PUF proteins, named for PUM (Pumilio) and FBF (fem-3 binding factor), are an exemplary system for understanding the divergence of RNA recognition within eukaryotic RNA-binding protein families. Eight PUM repeats are arranged in a crescent shape with the RNA bound on the concave face of the protein. Each repeat contributes a trio of amino acid residues, termed a tripartite recognition motif (TRM), that directly contact the opposing RNA base. FBF recognizes a 9-nt motif, 5´-UGURNNAUA-3´, whereas PUF-8 binds an 8-nt sequence, 5´-UGUANAUA-3´.

A crystal structure of the AS/Y variant in complex with PBE RNA was nearly identical to the SS/Y structure. We also tested the binding preferences of an FBF-2 R5 AQ/Y variant that we identified as an in vivo substitution by genome engineering (see below). We did, however, recover multiple strains with deletion mutations and a single strain that incorporated a novel repeat R5 TRM variant - AQ/Y. This mutant strain was designated fbf-2(lot14). Serendipitously the AQ/Y mutation preferentially binds to the PBE relative to the FBE in cells and in vitro, and a crystal structure of the FBF-2 R5 AQ/Y variant bound to the PBE adopts a similar conformation to SS/Y and AS/Y bound to the PBE. The R5 AQ/Y variant displayed preference for A4, although not as strictly as PUF-8. The AQ/Y variant is most similar to the WT TRM, which seems to impart preference for A4. Finally, the FBF-2 R5 AQ/Y variant demonstrates a recognition pattern qualitatively more similar to PUF-8 than FBF-2. In the case of changing specificity of FBF-2 to that of PUF-8, we have demonstrated that a minimum of two amino acid changes (CQ/R to AQ/Y) can swap binding element length preference, but they do not impact curvature. We found that the edited strain expressing the FBF-2 AQ/Y variant (fbf-2(lot-14), glp-1(ar202) animals) displayed tumor formation in only 36% of gonads at 15°C. Thus, the FBF-2 AQ/Y variant is capable of substituting for PUF-8 in vivo.

> GSNNVLPTWSLDSNGEMRSRLSLSEVLDSGDLMKFAVDKTGCQFLEKAVKGSLTSYQKFQLFEQVIGRKDDFLKLSTNIFGNYLVQSVIGISLATNDDGYTKRQEKLKNFISSQMTDMCLDKFACRVIQSSLQNMDLSLACKLVQALPRDARLIAICVDQNANHVIQKVVAVIPLKNWEFIVDFVATPEHLRQICSDKYGAYVVQTIIEKLTADSMNVDLTSAAQNLRERALQRLMTSVTNRCQELATNEYANYIIQHIVSNDDLAVYRECIIEKCLMRNLLSLSQEKFASHVVEKAFLHAPLELLAEMMDEIFDGYIPHPDTGKDALDIMMFHQFGNYVVQCMLTICCDAVSGRRQTKEGGYDHAISFQDWLKKLHSRVTKERHRLSRFSSGKKMIETLANLRSTHPIYELQ> GSLKIAPANADFAFRFYYLIASETPGKNIFFSPLSISAAYAMLSLGACSHSRSQILEGLGFNLTELSESDVHRGFQHLLHTLNLPGHGLETRVGSALFLSHNLKFLAKFLNDTMAVYEAKLFHTNFYDTVGTIQLINDHVKKETRGKIVDLVSELKKDVLMVLVNYIYFKALWEKPFISSRTTPKDFYVDENTTVRVPMMLQDQEHHWYLHDRYLPCSVLRMDYKGDATVFFILPNQGKMREIEEVLTPEMLMRWNNLLRKRNFYKKLELHLPKFSISGSYVLDQILPRLGFTDLFSKWADLSGITKQQKLEASKSFHKATLDVDEAGTEAAAATS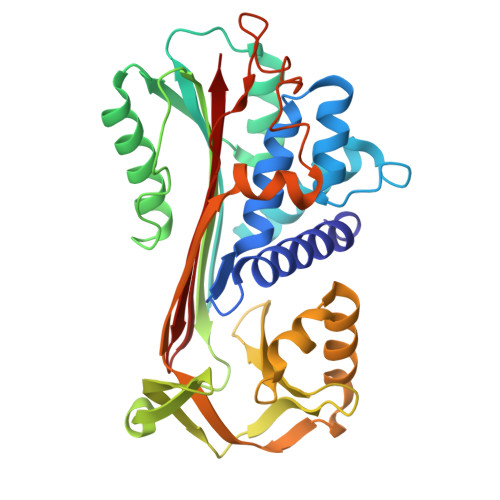FAIKF> MRFDNAAPPPPPPPEAAGSTTTSSSTAASALPRVSYRTLPSSMYPKEVSSDFIPFPLPKHDASMGFGPVRLRNVPDIEEARARMAKAAQGPPRGSASTQLQDADGDNAEAASALWAELSGETTATSVGLSTTSVTGASPEDPEALSRPPDAQDEDLVGYHVHRHFPLLDVLGCDRSVNDLLAQFWNRPQREARTATVLDFAATLQRHSNEELTRVLYELSSLFEWDGNGLQFIAAKVLKYGRSYTVSSELTKAFVQLVDAMTVAFVEEQPHRLAESPALLAQVLHFLALVKIMEPNKWYTLNPNAPQNRADYTHPRGVNRTCGHVTTGRALLDFLEDMVTSGHNWTGEAAVDDQQGSLARSPVPQHATNRFTEGWSEDDILDVMAGFSGVMPDGKASSPVLYALLDELWMRWSKVGFVLSGSEQAVRLERLYMLLQVMDMQRDAVLDALLGGQLRAHSTAPSTSTLPTLFCERDDTPPLTLAQSLTQTRGPDFFSAVSRDKRAMVKAAALRLLTASLAKARDDSDAVLHQALVESGTELLQSLTSKSAALSFAQREQFDVITLRAVPHMADVAERLAEQRAEAPFFPLTASAGGLPDTAAVLAHLSSHPAPYIVLCKGRRVHPVRTLVSNLDHVAAVENVFLLHSSGVSKCVDALVAVARRLRSGKDALIVTASCLRALQAAAQYGATEKRRATADRALDIVSYELEAGRAILMPVTDELYLHDAGTYCDEDLMLWTLAAYLARDVPLVKVHTIMSSRSRARNPQHALRGEHSPLTSTDDLYNKSTPLLQALRSKELRAVTHHPVVQRPVRDPPQTLYNVNPIRARFVYRRDK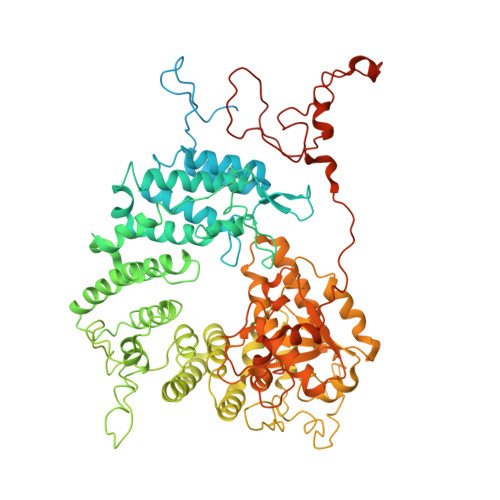ALFDKYHVTARNLAPGFSQGALNSDLRALGFYTPDHPQVPYTPLSELKCHPVPANPPASQ>TACRKHELYVSFQDLGWQDWIIAPKGYAANYCDGECSFPLNAHMNATNHAIVQTLVHLMNPEYVP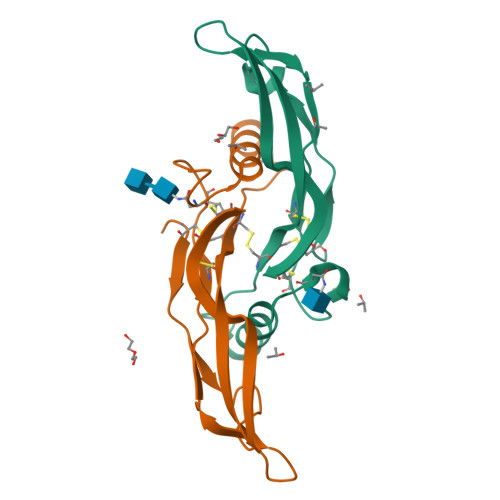KPCCAPTKLNAISVLYFDDNSNVILKKYRNMVVRACGCH[2x]In the Siphoviridae SPP1 phage, the tail tube consists of the TTPs gp17.1 and gp17.1* in a ratio of 3:1, with the latter being generated by a translational frameshift adding a fibronectin type III (FN3) domain to the C-terminus of the protein. However, virions only containing gp17.1 are still viable and infectious, indicating that the additional C-terminal FN3 domain is dispensable for phage assembly and infection. gp17.1 monomers are unstable in solution and spontaneously self-polymerize into long tubes in vitro which are indistinguishable from native tubes. Six gp17.1 subunits assemble into a ring with the inner 24 β-strands forming a β-barrel that defines the inner lumen of the tube. The α-helices are arranged almost parallel to the tail tube axis. These rings stack onto each other with a rotation of 21.9° forming a right-handed helical, hollow tube.

In this work, we set out to expand the labeling strategy for long-range distance restraints to further methyl groups, as well as to integrate the NMR data with a 3.5–6 Å cryo-EM map for hybrid structure calculation. For the collection of solid-state NMR long-range distance restraints, we overexpressed a set of differently labeled TTP gp17.1 in E. coli, purified them, and let them self-polymerize into native-like tail tubes as detailed in the “Methods” section. Torsion angles were predicted based on assigned backbone chemical shifts. Hence, these samples deliver a set of restraints that defines the relative organization of gp17.1 subunits within the tube. During structure calculation only the structure of a single monomer was represented and refined. The structures of the other subunits were generated by applying symmetry operators to the subunit structure. We represented two stacked rings in the structure calculation. Each ring was composed of six subunits such that interactions between twelve subunits were considered in the structure calculation.

>[12x]PIMGQDVKYLFQSIDAATGSAPLFPAYQTDGSVSGERELFDEQTKNGRILGPGSVADSGEVTYYGKRGDAGQKAIEDAYQNGKQIKFWRVDTVKNENDKYDAQFGFAYIESREYSDGVEGAVEISISLQVIGELKNGEIDTLPEEIVNVSKGGYDFQQPGQTTGEAPGTVPA> MGMEMDKNLVREVIAKRVAQEFHDGYVVNLGIGLPTLVANYVGDMDVIFQSENGCIGVGPAPEKGKEDPYLVNAG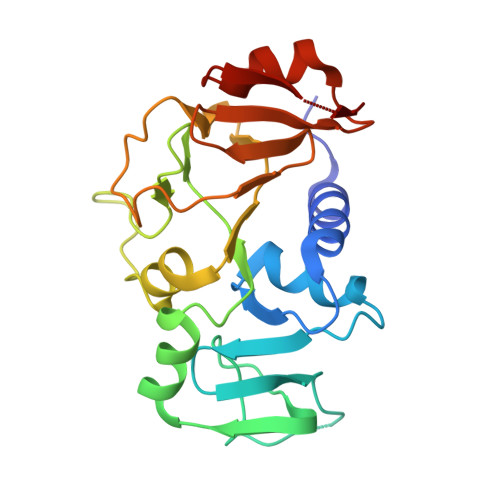AGFITAAKGAMFFDSAYSFGIIRGGHVDATVLGALEVDEKGNLANWMIPGKKVPGMGGAMDLVVGAKKVIVAMEHTSNGAIKILKECKLPLTAVGVVDLIITEKAVFEVTDKGLVLKEITPYSSLEDIKATTAADFIIADDLKK>SSSAMPDVPAPLTNLQFKYTKIFINNEWHSSVSGKKFPVFNPATEEKLCEVEEGDKEDVDKAVKAARQAFQIGSPWRTMDASERGRLLNKLADLIERDRLLLATMEAMNGGKLFSNAYLMDLGGCIKTLRYCAGWADKIQGRTIPMDGNFFTYTRSEPVGVCGQIIPWNFPLLMFLWKIGPALSCGNTVVVKPAEQTPLTALHMGSLIKEAGFPPGVVNIVPGYGPTAGAAISSHMDVDKVAFTGSTEVGKLIKEAAGKSNLKRVSLELGGKSPCIVFADADLDNAVEFAHQGVFYHQGQCCIAASRLFVEESIYDEFVRRSVERAKKYVLGNPLTPGVSQGPQIDKEQYEKILDLIESGKKEGAKLECGGGPWGNKGYFIQPTVFSDVTDDMRIAKEEIFGPVQQIMKFKS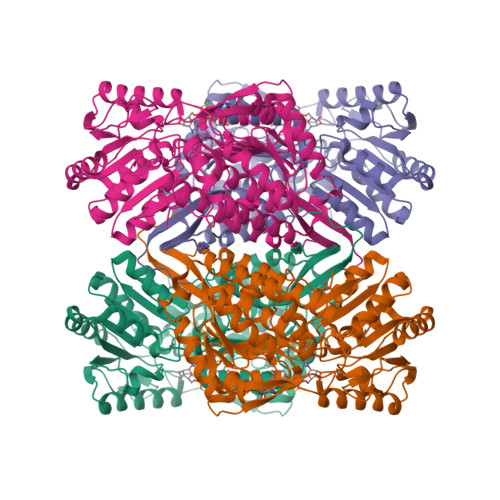LDDVIKRANNTFYGLSAGIFTNDIDKAITVSSALQSGTVWVNCYSVVSAQCPFGGFKMSGNGRELGEYGFHEYTEVKTVTIKISQKNS[4x]> P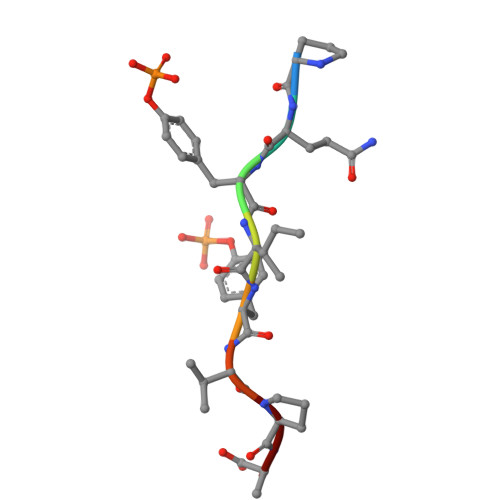QYIYVPA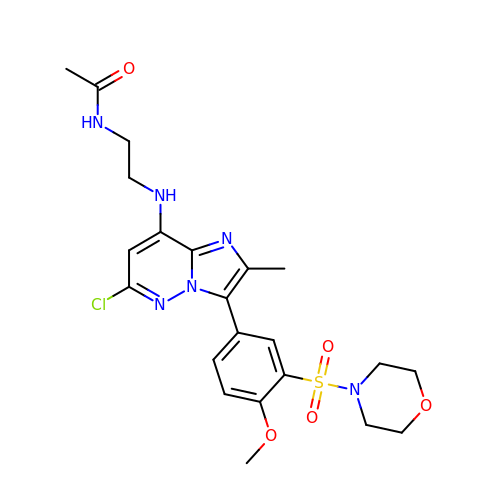~{N}-[2-[[6-chloranyl-3-(4-methoxy-3-morpholin-4-ylsulfonyl-phenyl)-2-methyl-imidazo[1,2-b]pyridazin-8-yl]amino]ethyl]ethanamide | C22 H27 Cl N6 O5 S | YJBQUXYOUNYKNC-UHFFFAOYSA-N>MQPVLVFKLTADFREDPDPRKVNLGVGAYRTDDCHPWVLPVVKKVEQKIANDNSLNHEYLPILGLAEFRSCASRLALGDDSPALKEKRVGGVQSLGGTGALRIGADFLARWYNGTNNKNTPVYVSSPTWENHNAVFSAAGFKDIRSYRYWDAEKRGLDLQGFLNDLENAPEFSIVVLHACAHNPTGIDPTPEQWKQIASVMKHRFLFPFFDSAYQGFASGNLERDAWAIRYFVSEGFEFFCAQSFSKNFGLYNERVGNLTV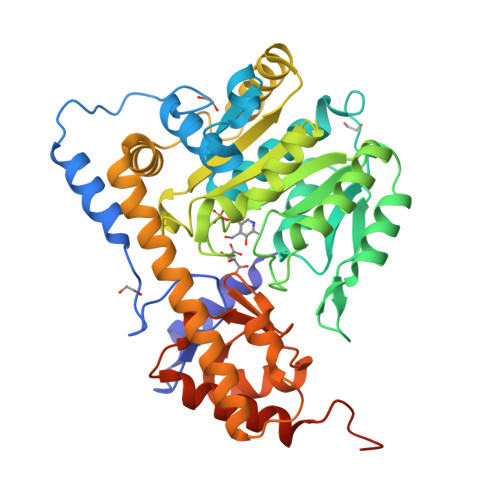VGKEPESILQVLSQMEKIVRITWSNPPAQGARIVASTLSNPELFEEWTGNVKTMADRILTMRSELRARLEALKTPGTWNHITDQIGMFSFTGLNPKQVEYLVNEKHIYLLPSGRINVSGLTTKNLDYVATSIHEAVTKIAENLYFQSHHHHHHDYKDDDDK[4x]>[2x]SMSKNNIFNKYPTIIHGEARGENDEFVVHTRYPRFLARKSFDDNFTGEMPAKPVNGELGQIGEPRRLAYDSRLGLWLSDFIMLDNNKPKNMEDWLGQLKAACDRIAADDL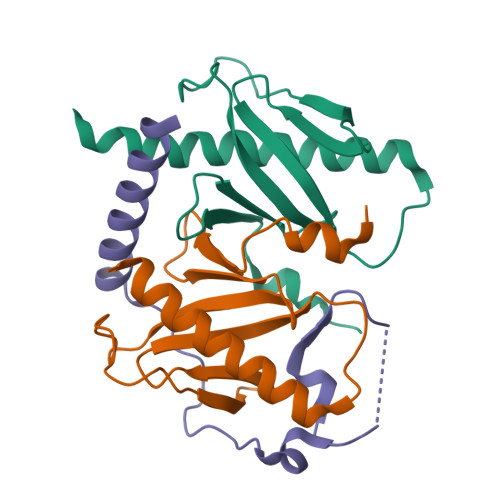MLNEDAADLEGWDD;> SMAAFKPNSINYILGLDIGIASVGWAMVEIDEEENPIRLIDLGVRVFERAEVPKTGDSLAMARRLARSVRRLTRRRAH> VQFYWLDLYGILGENLDIQNFLPLETSKFKSLTSEYKMITTRAFQLDTTIEVIHIPNFDTTLKLTIDSLKMIKSSLSTFLERQRRQFPRFYFLGNDDLLKIIGSGKHHDQVSKFMKKMFGSIESIIFFEDSITGVRSVEGEVLNLNEKIELKDSIQAQEWLNILDTEIKLSVFTQFRDCLGQLKDGTDIEVVVSKYIFQAILLSAQVMWTELVEKCLQTNEFSKYWKEVDMKIKGLLDKLNKSSDNVKKKIEALLVEYLHFNNVIGQLKNCSTKEEARLLWAKVQKFYQKNDTLDDLNSVFISQSGYLLQYKFEYIGIPERLIYTPLLLVGFATLTDSLHQKYGGCFFGPAGTGKTETVKAFGQNLGRVVVVFNCDDSFDYQVLSRLLVGITQIGAWGCFDEFNRLDEKVLSAVSANIQQIQNGLQVGKSHITLLEEETPLSPHTAVFITLNPGYNGRSELPENLKKSFREFSMKSPQSGTIAEMILQIMGFEDSKSLASKIVHFLELLSSKCSSMNHYHFGLRTLKGVLRNCSPLVSEFGEGEKTVVESLKRVILPSLGDTDELVFKDELSKIFDSAGTPLNSKAIVQCLKDAGQRSGFSMSEEFLKKCMQFYYMQKTQQALILVGKAGCGKTATWKTVIDAMAIFDGHANVVYVIDTKVLTKESLYGSMLKATLEWRDGLFTSILRRVNDDITGTFKNSRIWVVFDSDLDPEYVEAMNSVLDDNKILTLPNGERLPIPPNFRILFETDNLDHTTPATITRCGLLWFSTDVCSISSKIDHLLNKSYEALDNKLSMFELDKLKDLISDSFDMASLTNIFTCSNDLVHILGVRTFNKLETAVQLAVHLISSYRQWFQNLDDKSLKDVITLLIKRSLLYALAGDSTGESQRAFIQTINTYFGHDSQELSDYSTIVIANDKLSFSSFCSEIPSVSLEAHEVMRPDIVIPTIDTIKHEKIFYDLLNSKRGIILCGPPGSGKTMIMNNALRNSSLYDVVGINFSKDTTTEHILSALHRHTNYVTTSKGLTLLPKSDIKNLVLFCDEINLPKLDKYGSQNVVLFLRQLMEKQGFWKTPENKWVTIERIHIVGACNPPTDPGRIPMSERFTRHAAILYLGYPSGKSLSQIYEIYYKAIFKLVPEFRSYTEPFARASVHLYNECKARYS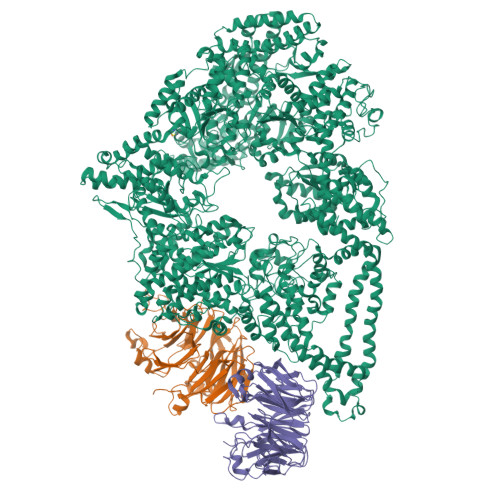TGLQSHYLFSPRELTRLVRGVYTAINTGPRQTLRSLIRLWAYEAWRIFADRLVGVKEKNSFEQLLYETVDKYLPNQDLGNISSTSLLFSGLLSLDFKEVNKTDLVNFIEERFKTFCDEELEVPMVIHESMVDHILRIDRALKQVQGHMMLIGASRTGKTILTRFVAWLNGLKIVQPKIHRHSNLSDFDMILKKAISDCSLKESRTCLIIDESNILETAFLERMNTLLANADIPDLFQGEEYDKLLNNLRNKTRSLGLLLDTEQELYDWFVGEIAKNLHVVFTICDPTNNKSSAMISSPALFNRCIINWMGDWDTKTMSQVANNMVDVVPMEFTDFIVPEVNKELVFTEPIQTIRDAVVNILIHFDRNFYQKMKVGVNPRSPGYFIDGLRALVKLVTAKYQDLQENQRFVNVGLEKLNESVSLTFEKERWLNTTKQFSKTSQELIGNCIISSIYETYFGHLNERERGDMLVILKRLLGKFAVKYDVNYRFIDYLVTLDEKMKWLECGLDKNDYFLENMSIVMNSQDAVPFLLDPSSHMITVISNYYGNKTVLLSFLEEGFVKRLENAVRFGSVVIIQDGEFFDPIISRLISREFNHAGNRVTVEIGDHEVDVSGDFKLFIHSCDPSGDIPIFLRSRVRLVHFVTNKESIETRIFDITLTEENAEMQRKREDLIKLNTEYRLKLKNLEKRLLEELNNSQGNMLENDELMVTLNNLKKEAMNIEKKLSESEEFFPQFDNLVEEYSIIGKHSVKIFSMLEKFGQFHWFYGISIGQFLSCFKRVFIKKSRETRAARTRVDEILWLLYQEVYCQFSTALDKKFKMIMAMTMFCLYKFDIESEQYKEAVLTMIGVLSESSDGVPKLTVDTNDDLRYLWDYVTTKSYISALNWFKNEFFVDEWNIADVVANSENNYFTMASERDVDGTFKLIELAKASKESLKIIPLGSIENLNYAQEEISKSKIEGGWILLQNIQMSLSWVKTYLHKHVEETKAAEEHEKFKMFMTCHLTGDKLPAPLLQRTDRVVYEDIPGILDTVKDLWGSQFFTGKISGVWSVYCTFLLSWFHALITARTRLVPHGFSKKYYFNDCDFQFASVYLENVLATNSTNNIPWAQVRDHIATIVYGGKIDEEKDLEVVAKLCAHVFCGSDNLQIVPGVRIPQPLLQQSEEEERARLTAILSNTIEPADSLSSWLQLPRESILDYERLQAKEVASSTEQLLQEM;>[2x]LKWIPRNLPSCLINVESSVTSVKLHPNLPIVFVATDHGKLYAFDLFNYTIPLASLQSHTKAITSMDVLFTNYTNSSKKNYLVIVTASKDLQIHVFKWVSEECKFQQIRSLLGHEHIVSAVKIWQKNNDVHIASCSRDQTVKIWDFHNGWSLKTFQPHSQWVRSIDVLGDYIISGSHDTTLRLTHWPSGNGLSVGTGHEFPIEKVKFIHFIEDSPEIRFRTPSTDRYKNWGMQYCVSASRDRTIKIWEIPLPTLMAHRAPIPNPTDSNFRCVLTLKGHLSWVRDISIRGQYLFSCADDKSVRCWDLNTGQCLHVWEKLHTGFVNCLDLDVDFDSNVTPRQMMVTGGLDCKSNVFM>[2x]MSLTFSILAHDPETG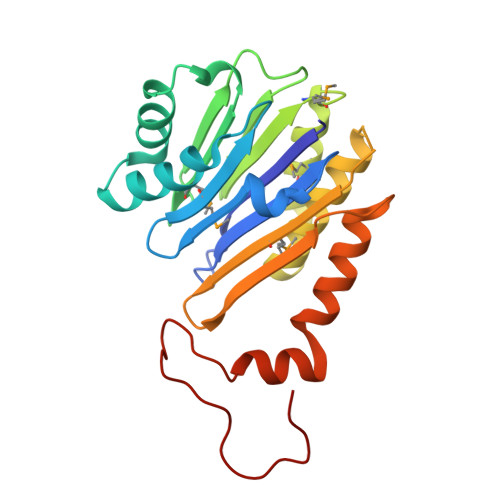AIGGAAATGSLCVGGWVLRGDLNAGMSASQGAAPSTFWGEEVLQHLRDGSHPEDAVNHVTSQDSGRAYRQLAAMDLLGNAAAFTGSENQDIKGSVTFASGIASGNMLGDNSVLGAMTEAFVASDLTFERRLLAALIAAEGAGSDFRGLLSAAMLVLHPDRPPVTLRIDYHPDNPIGALEQLYQKATTGDYADWARQVPVLSDKERILDEGHHHHHH>[2x]AHGRIELIIGPMFAGKTTELMRRV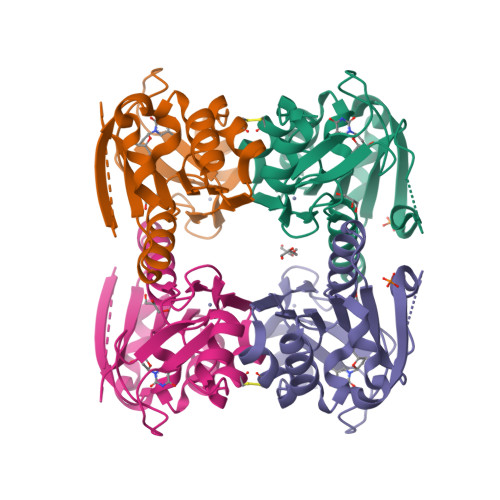QRHKHAQRSCYIIKYTGDTRYSEGAITSHDQRALTANVSVSNLHDVGDEWRKYDVIAVDEGQFFPDVAAFCSKAADSGKVVIVSALDADYLQEPFEEICLLVSRADSVVKLSAVCMECHNRKASFTYRTVKSDERKLVGGSDMYMSVCRSCYETKRNM> LKAL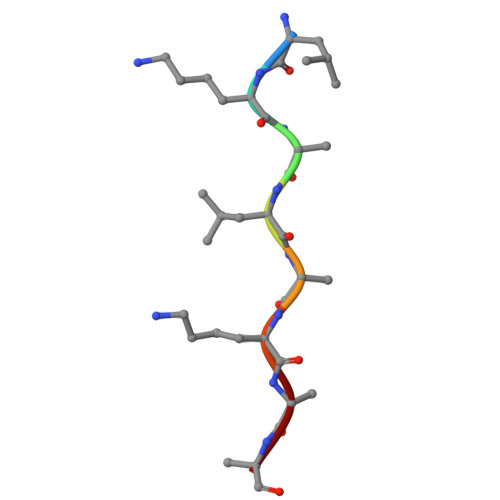KKLA>MGGEVEEPEPQMVLSPLTSAAIFLVVTIDSGGEDTVRDLLSDVASLERAVGFRAQPDGRLSCVTGIGSEAWDRLFSGARPAGLHPFRELDGPVHRAVATPGDLLFHIRASRLDLCFALATEIMGRLRGAVTPQDEVHGFKYFDERDMLGFVDGTENPTGAAARRAVLVGAEDPAFAGGSYAVVQKYLHDIDAWEGLSVEAQERVIGRRKMTDVELSDDVKPADSHVALTSVTGPDGSDLEILRDNMPFGSVGREEFGTYFIGYARTPEVTETMLERMFLGTASAPHDRILDFSTAVTGSLFFTPAADFLEDLSARP[6x]

Dye‐decolorising peroxidases (DyPs) are the most recent member of the peroxidase family to be discovered. Three DyPs have been identified in S. lividans; two A‐types (DtpA and DtpAa) and one B‐type (DtpB). Using serial femtosecond X‐ray crystallography (SFX), we have determined the pristine structures of the FeIII and FeIV=O redox states of a B‐type DyP. These structures reveal a water‐free distal heme site that, together with the presence of an asparagine, imply the use of the distal arginine as a catalytic base.

A composite compound I X‐ray structure at 100 K was determined in order to assess temperature effects on structure and further confirmed the presence of a short Fe−O bond of 1.65±0.17 Å in monomer A, with the mean distance in all six monomers being 1.76 Å. Fe−O bond lengths for compound I and II from several structures of nonmammalian peroxidases determined at 100 K are reported in Table 1, with the short Fe−O bond in DtpB most consistent with a compound I FeIV=O species. The heme redox state in the crystals was corroborated through analysis of larger DtpB crystals suitable to obtain electronic absorbance spectra at 100 K. Identical electronic absorbance bands to those for FeIII‐DtpB and compound I in solution were observed in the crystals. No further change in the electronic absorbance spectrum following addition of H2O2 to DtpB is observed for >1 h at room temperature (RT), indicating DtpB forms a highly stable compound I species.> TYGIRLRVWGDYACFTRPEMKVERVSYDVMPPSAARGILEAIHWKPAIRWIVDRIHVLRPIVFDNVRRNEVSSKIPKPNPATAMRDRKPLYFLVDDGSNRQQRAATLLRNVDYVIEAHFELTDKAGAEDNAGKHLDIFRRRARAGQSFQQPCLGCREFPASFELLEGDVPLSCYAGEKRDLGYMLLDIDFERDMTPLFFKAVMEDGVITPPSRTSPEVRA;>[7x]MTAIANRYEFVLLFDVENGNPNGDPDAGNMPRIDPETGHGLVTDVCLKRKIRNHVALTKEGAERFNIYIQEKAILNETHERAYTACDLKPEPKKLPKKVEDAKRVTDWMCTNFYDIRTFGAVMTTEVNCGQVRGPVQMAFARSVEPVVPQEVSITRMAVTTKAEAEKQQGDNRTMGRKHIVPYGLYVAHGFISAPLAEKTGFSDEDLTLFWDALVNMFEHDRSAARGLMSSRKLIVFKHQNRLGNAPAHKLFDLVKVSRAEGSSGPARSFADYAVTVGQAPEGVEVKEML;> WENTSYILGVDAKGKQERTDKCHAAFIAHIKAYCDTADQDLAAVLQFLEHGEKDLSAFPVSEEVIGSNIVFRIEGEPGFVHERPAARQAWANCLNRREQGLCGQCLITGERQKPIAQLHPSIKGGRDGVRGAQAVASIVSFNNTAFESYGKEQSINAPVSQEAAFSYVTALNYLLNPSNRQKVTIADATVVFWAERSSPAEDIFAGMFDPPSTTAKPESSNGTPPEDSEEGSQPDTARDDPHAAARMHDLLVAIRSGKRATDIMPDMDESVRFHVLGLSPNAARLSVRFWEVDTVGHMLDKVGRHYRELEIIPQFNNEQEFPSLSTLLRQTAVLNKTENISPVLAGGLFRAMLTGGPYPQSLLPAVLGRIRAEHARPEDKSRYRLEVVTYYRAALIKAYLIRNRKLEVPVSLDPARTDRPYLLGRLF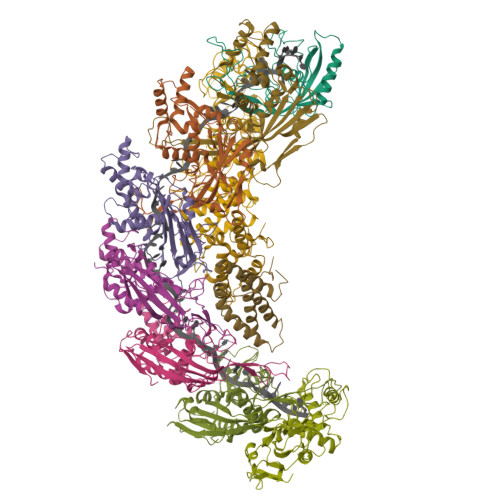AVLEKAQEDAVPGANATIKDRYLASASANPGQVFHMLLKNASNHTAKLRKDPERKGSAIHYEIMMQEIIDNISDFPVTMSSDEQGLFMIGYYHQRKALFTKKNKEN;>[2x]VSLDPARTDRPYLLGRLFAVLEKAQEDAVPGANATIKDRYLASASANPGQVFHMLLKNASNHTAKLRKDPERKGSAIHYEIMMQEIIDNISDFPVTMSSDEQGLFMIGYYHQRKALFTKKNKEN PHOSPHITE 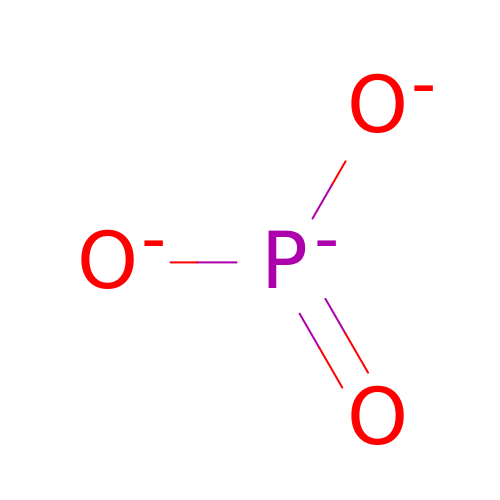ION | O3 P | AQSJGOWTSHOLKH-UHFFFAOYSA-N> MKHHHHHHPMACNFQFPEIAYPGKLICPQYGTENKDGEDIIFNYVPGPGT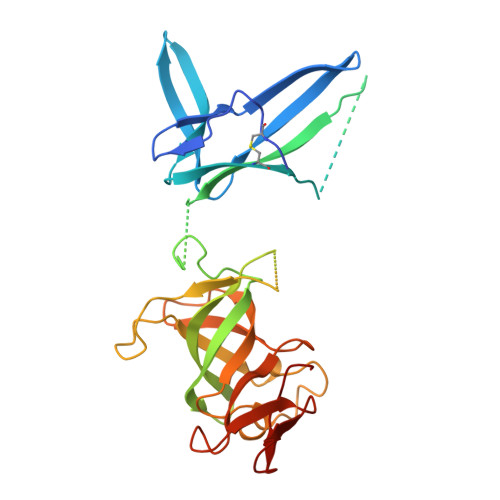KLIQYEHNGRTLEAITATLVGTVRCEEEKKTDQEEEREGTDQSTEEEKSVDASPNDVTRRTVKNILVSVLPGTEKGRKTNKYANNDFANNLPKEGDIVLTRVTRLSLQRANVEILAVEDKPSPIDSGIGSNGSGIVAAGGGSGAATFSVSQASSDLGETFRGIIRSQDVRSTDRDRVKVIECFKPGDIVRAQVLSLGDGTNYYLTTARNDLGVVFARAANGAGGLMYATDWQMMTSPVTGATEKRKCAKPF> SDKSG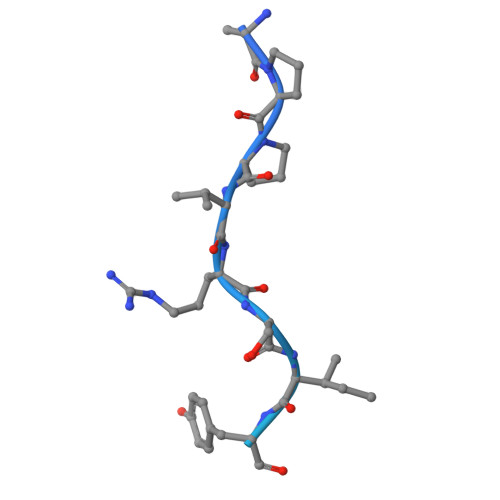APPVRSIYDDISSPGLGSTPLTSRRQPNISVMQSPLVGVTSTPGTGQSMFSPASIGQPRKTTL> SNAMQTVPSSDGTPIAFERSGSGPPVVLVGGALSTRAGGAPLAERLAPHFTVICYDRRGRGDSGDTPPYAVEREIEDLAAIIDAAGGAAFVFGMSSGAGLSLLAAASGLPITRLAVFEPPYAVDDSRPPVPPDYQTRLDALLAEGRRGDAVTYFMTEGVGVPPDLVAQMQQAPMWPGMEAVAHTLPYDHAVMGDNTIPTARFASISIPTLVMDGGASP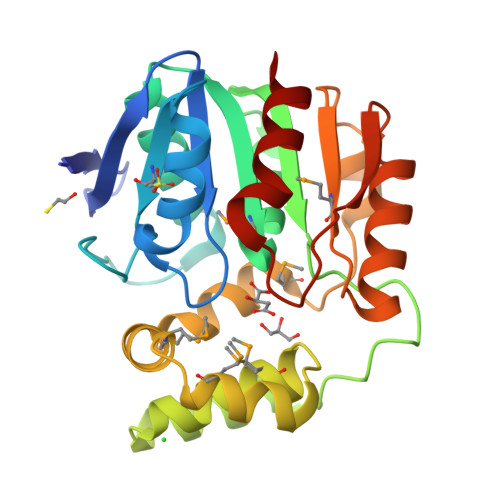AWIRHTAQELADTIPNARYVTLENQTHTVAPDAIAPVLVEFFTR>MEGVDLLGFLIITLNCNVTMVGKLWFVLTMLLRMLVIVLAGRPVYQDEQERFVCNTLQPGCANVCYDVFSPVSHLRFWLIQGVCVLLPSAVFSVYVLHRGATLAALGPRRCPDPREPASGQRRCPRPFGERGGLQV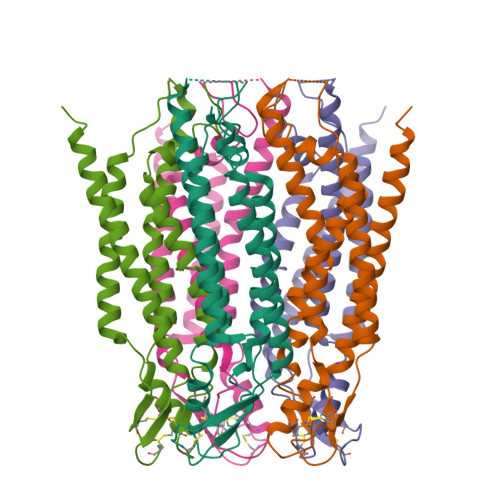PDFSAGYIIHLLLRTLLEAAFGALHYFLFGFLAPKKFPCTRPPCTGVVDCYVSRPTEKSLLMLFLWAVSALSFLLGLADLVCSLRRRMRRRPGPPTS[5x]>[2x]GHMALSLANYLAADSAAEALRRDVRAGLTATQKSLPPKWFYDAVGSDLFDQITRLPEYYPTRTEAQILRTRSAEIISAAGADTLVELGSGTSEKTRMLLDAMRDAELLRRFIPFDVDAGVLRSAGAAIGAEYPGIEIDAVCGDFEEHLGKIPHVGRRLVVFLGSTIGNLTPAPRAEFLST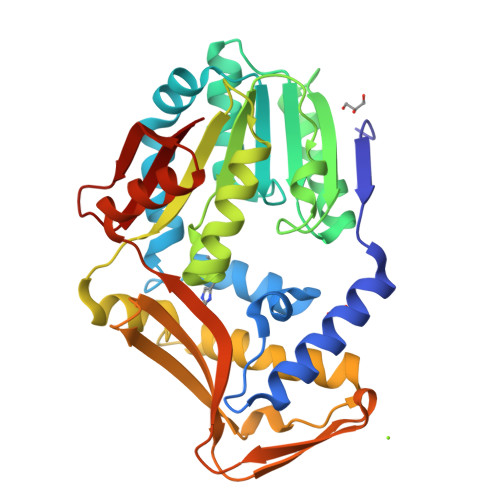LADTLQPGDSLLLGTDLVKDTGRLVRAYDDAAGVTAAFNRNVLAVVNRELSADFDLDAFEHVAKWNSDEERIEMWLRARTAQHVRVAALDLEVDFAAGEEMLTEVSCKFRPENVVAELAEAGLRQTHWWTDPAGDFGLSLAVR Here, we take a structural approach to assess the relatedness of these eukaryotic-like proteins in Asgard archaea, the closest known prokaryotic relatives to eukaryotes. Asgard archaea roadblock, longin and TRAPPC3 domain-containing proteins form dimers similar to those found in the eukaryotic TRAPP and Ragulator complexes. Here, we adopted an X-ray crystallography approach to compare the structures of a potential Asgard Rab small GTPase, several RBs and two TRAPPC3 proteins to their eukaryotic counterparts, with a focus on Thor and MKD1. We conclude that the emergence of these protein architectures predated eukaryogenesis, however further adaptations occurred in proto-eukaryotes to allow these proteins to regulate distinct internal membranes.

The proteins (Thor-RB and MKD1-RB) were purified, crystallized and their structures were elucidated via X-ray crystallography to 2.14 and 2.69 Å, respectively. Both proteins are homodimers formed from protomers comprised of 5-stranded β-sheets sandwiched between a single α-helix (formed between strands 2 and 3) and a pair of α-helices (formed from the N- and C-termini). We compared the structural similarities of Thor-RB and MKD1-RB with MglBs and eukaryotic RB proteins. Both proteins displayed approximately similar levels of homology with the RB proteins M. xanthus MglB and H. Sapiens LAMTOR2, matching ~110 residues with an RMSD of 1.5–1.6 Å. Lower levels of homology were seen in comparison with longin domains (86–94 residues, RMSD of 2.5-3.0 Å) and profilins (96–102 residues, RMSD of 1.7–2.7 Å). These homologies indicate that the RB fold is highly conserved between all domains of life and that the profilin and longin domains share a core structure with RB. Despite the similarity in structures, Thor-RB and MKD1-RB display different surface charge distributions. Thus, we hypothesize that MKD1-RB may be a membrane-interacting module, whereas Thor-RB, which lacks the basic patch, may be a scaffold protein for protein:protein interactions. The Odin-RBLC7 structure shares a similar homodimeric structure to Thor-RB and MKD1-RB but lacks the terminal pair of α-helices observed in the RB structures.

>[6x]MSSAVDNINKTIRDFETVPGVEGAALVSADGLMISSALPETEQERVAAISAGLLSLGEKATTELDRGNFKEVYVKGEKGYTLLTSVGENALLLVLAKADAQIGLIFVDMRRIADSLLEIL>SGPGFDFAQAIMKKNTVIARTEKGEFTMLGVYDRVAVIPTHASVGETIYINDVETKVLDACALRDLTDTNLEITIVRLDRNQKFRDIRHFLPRYEDDYNDAVLSVHTSKFPNMYIPVGQVTNYGFLNLGGTPTHRILMYNFPTRAGQAGGVVTTTGKVIGIHVGGNGAQGFAAMLLHSYFSD[2x];> AKVQGP

During viral replication of EV68, the viral genome is translated into a single, large polyprotein comprised of structural and non-structural proteins. The viral polyprotein needs to be cleaved into individual proteins for viral replication to proceed. The 3C protease cleaves eight sites in the polyprotein with a preference for a glutamine–glycine (QG) motif at the P1/P1′ positions. The conserved essential function in viral replication makes the 3C protease a promising target for DAA development.

While the co-crystal structures of EV68-3C protease with viral substrates had remained elusive, we have solved and refined the first such co-crystal structure. Superposition of these two structures, experimental and computational, revealed a very good agreement with the converged modeled substrate peptide position, and the peptide from the experimental crystal structure fits well within the substrate envelope. However, once the peptide binds, the pocket becomes capped off, enclosing the P1 glutamine peptide in a U-shaped pocket. Specifically, the Thr142 sidechain is shifted 3.6 Å deeper into the S1 pocket, opening that area for a water molecule to coordinate with the backbones of Gln168, Gly166, and Asn165. At the same time, Thr142 is positioned closer to the P1 glutamine, enabling the Thr142 hydroxyl to form a hydrogen bond with the incoming substrate peptide. Proximal to the structural water, we observed a 4.3 Å conformational change of Arg143 to form a hydrogen bond with Gly166 that is unique to the substrate-bound structure forming the S1 pocket. Compared to the apo protease, loop 125–129 retained its overall shape but was closer to the P3 and P4 region of the substrate in the bound structure. For the substrate-bound protease, Asn126 in this loop was 0.7 Å closer to the peptide, enabling a hydrogen bond. Similarly, Gly128 was 1.3 Å closer to the P4 backbone nitrogen in the substrate-bound structure, facilitating another hydrogen bond interaction.>QDSTSDLIPAPPLSKVPLQQNFQDNQFHGKWYQVGRAGNAALREDKDPQKMTAQIYELKEDKSYNVTAVRFRKKKCDYLTMTFVPGSQPGEFTLGNIKSYPGLTSYLVRVVSTNYNQHAMVFFKKVSQNREYFSITLLGRT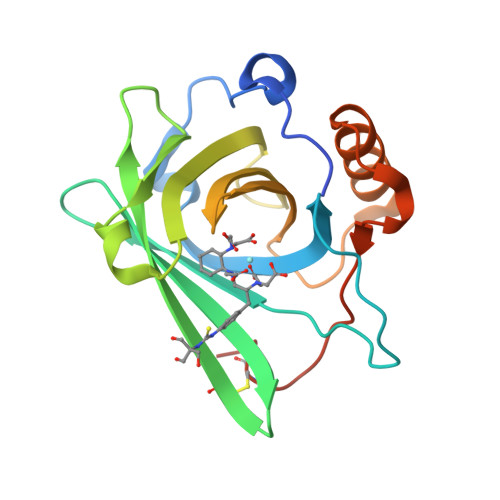KELASELKENFIRFSKSLGLPENHIVFPVPIDQCIDGSAHHHHHH[2x]>[16x]AKDKEFQVLFVLTILTLISGT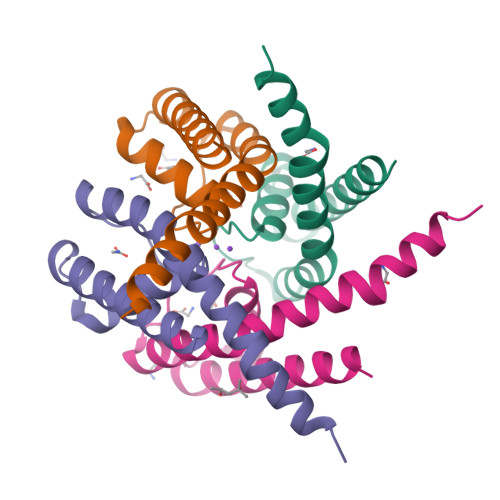IFYSTVEGLRPIDALYFSVVTLTTVGEAPPPQTDFGKIFTILYIFIGIGLVFGFIHKLAVNVQLPSILSNVVP5'-{[(2-amino-3-hydroxybenzene-1-carbonyl)sulfamoyl]amino}-5'-deoxyadenosine | C17 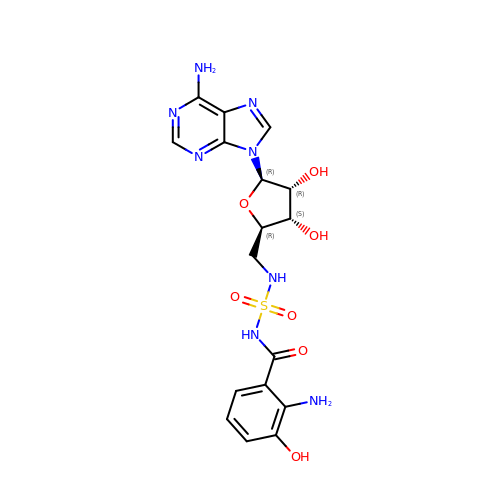H20 N8 O7 S | CBVBTJCJEIYIFL-DMEFTLKTSA-N> SGIRELNLTKEQHEWLNGWLELWGAWVYSGRLEKRMSSVIAKFMESVEPGRVMTRPMCN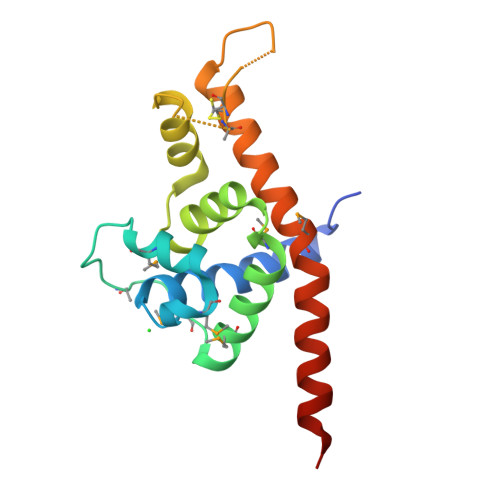DDDGMLISQVVDSVMYIDKKAFGILLSYYAHGSSKHAIASYYHRVARPRKMLCRGGGRIQKPSLATCRREVDEILNASLFMIYPVLDSAFKNRKRVEKIKHVA>[4x]SMGQETSYIEDNCNQNGAISLIFSLKEEVGALAKVLRLFEENDVNLTHIESRPSRLKKDEYEFFTHLDKRSLPALTNIIKILRHDIGATVHELSRDKKKDTV

Phenylalanine hydroxylase (PAH; EC 1.14.16.1) catalyzes the first step of l-phenylalanine (Phe) degradation via its hydroxylation to l-tyrosine, and serves to metabolize excess Phe in the diet. Like other AAAHs, PAH adopts a multi-domain architecture comprised of an N-terminal regulatory domain (RD, ~100 aa), a central catalytic domain (CD, ~300 aa) and a C-terminal multimerization helix (MH, ~40 aa). PAH-RD contains an ACT (Aspartate kinase, Chorismate mutase and TyrA) fold commonly found in enzymes for binding small molecule ligands. Some, if not all, of these regulatory properties are likely mediated by the N-terminal RD, as deletion of the domain liberates the enzyme from activation and renders it constitutively active.

In this study, we have determined the high resolution crystal structure of human PAH-RD bound with Phe. Trypsin-treated hPAH-RD19–118 yielded diffraction-quality crystals in the presence of Phe, allowing its structure determination at 1.8 Å resolution. In the final model, the peptide regions Gly19-Gly33 and Asp112-Val118 are not present, which can be due to intrinsic disorder, or possible trypsinization, of the two regions. The structure of hPAH-RD is a homodimer, with two βαββαβ folds (one from each protomer) arranged side-by-side to form a continuous 8-stranded β-sheet, resulting in an internal 2-fold symmetry. The dimer interface is largely polar in nature, comprising main-chain/side-chain hydrogen bonds contributed from two amino acid regions Glu43-Leu48 and Asn61-Ser67, as well as from a bound Phe ligand. Omit Fo-Fc electron density map revealed two Phe molecules bound to the hPAH-RD homodimer, at the interface of the two βαββαβ folds along the plane of the 2-fold axis (inset). Each Phe binding site comprises residues from both protomers, including the ‘ExVxAL’ (aa 43–48) and ‘YxF’ (aa 77–79) sequence regions of one protomer, and the ‘NLTIxS’ (aa 61–67) region of the other. Significant Cα differences (RMSD >2 Å) between the two structures are found, and regions that undergo most conformational changes in the presence of Phe include: (i) loop L1 and the first turn of helix α1 (aa 42–49), which brings in residues of the ‘ExVxAL’ motif for Phe binding, and (ii) the segment (aa 59–75) containing loop L2, strand β2 and loop L3, which is displaced outwards to ‘open up’ the Phe-binding site. The key finding of our study is that the binding of Phe to PAH-RD restructures the ACT fold, forming the necessary inter-subunit dimer interface and the resultant Phe allosteric site. To reconcile the difference with the recently reported rat PAH full-length structure, which did not reveal ACT:ACT interactions in the unliganded form12, we propose that the rat full-length PAH structure in the absence of Phe and our human PAH-RD structure in the presence of Phe could represent the unliganded ‘active-site blocking mode’ and the Phe-bound ‘multimerization mode’ of the domain, respectively.>[2x]METFTVKMGADSGLL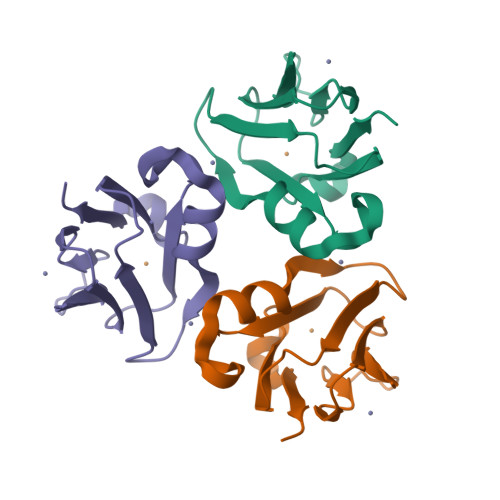QFEPANVTVHPGDTVKWVNNKLPPHNILFDDKQVPGASKELADKLSHSQLMFSPGESYEITFSSDFPAGTYTYYCAPHRGAGMVGKITVEG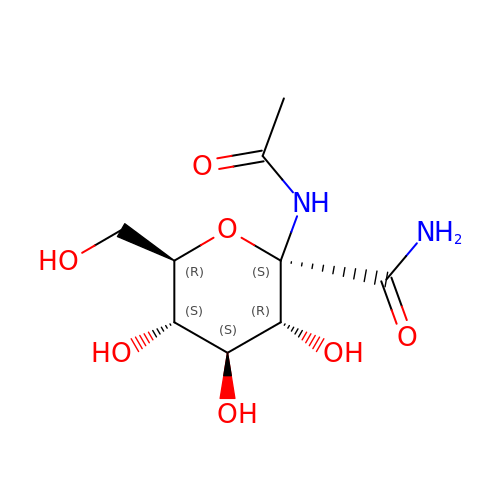1-DEOXY-1-ACETYLAMINO-BETA-D-GLUCO-2-HEPTULOPYRANOSONAMIDE | C9 H16 N2 O7 | BUPVODXECQDZQR-YCOWOFQRSA-N The hexanucleotide repeat expansion, GGGGCC (G4C2), within the first intron of the C9orf72 gene is known to be the most common genetic cause of both amyotrophic lateral sclerosis (ALS) and frontotemporal dementia (FTD). The G4C2 repeat expansions, either DNA or RNA, are able to form G-quadruplexes which induce toxicity leading to ALS/FTD. Here, we present the first crystal structures of an eight-layer parallel tetrameric G-quadruplex formed by two repeats of C9orf72 HRE DNA, d(G4C2)2, in Ba2+ and K+ solution, named as d(G4C2)2-Ba and d(G4C2)2-K respectively. Two d(G4C2)2 oligonucleotides form a parallel propeller-type dimeric G-quadruplex which stacks in a 5′-to-5′ arrangement making up a tetramer.

The crystal structure of d(G4C2)2-Ba in C2221 space group was solved by Ba-SAD method to 1.60 Å resolution. For the structure of d(G4C2)2-Ba (C2221), the asymmetric unit contains six chains, A–F. Intriguingly, two d(G4C2)2 oligonucleotides form a parallel-stranded dimeric G-quadruplex unit (i.e. chains A/B, chains C/D, chains E/F) which is composed of four G-tetrads connected by two CC double-chain-reversal loops. Specifically, chains A/B and their crystallographically symmetric molecules (chains Asym/Bsym) form a parallel-stranded tetrameric eight-layer G-quadruplex termed as Form-1/7 with the G1 base in one dimeric block stacks (i.e. chains A/B) with the G7 base in the opposite dimeric block (i.e. chains Asym/Bsym). While another two identical parallel-stranded tetrameric G-quadruplexes are formed by the chains C/D with their crystallographically symmetric molecules (chains Csym/Dsym) or chains E/F with their crystallographically symmetric molecules (chains Esym/Fsym). Both of them are named as Form-1/1 as the G1 base of one dimeric block (i.e. chains C/D or chains E/F) stacks on the G1 base of another dimeric block (i.e. chains Csym/Dsym or chains Esym/Fsym). The electron density was well defined for the four equal-spaced Ba2+ ions lying along the axis within the central core of the eight-layer tetrameric G-quadruplex in Form-1/7 and Form-1/1. Each of them is coordinated to eight neighbouring guanine O6 atoms at a distance of ∼2.7 Å, featuring an anti-prismatic coordination environment, which mimics those of monovalent potassium ions in DNA G-quadruplexes. Interestingly, an additional Ba2+ ion is positioned between two adjacent dimeric G-quadruplexes (formed by chains A/B and chains C/D, respectively) in the asymmetric unit. Interestingly, the C11 and C12 bases from two isolated chains, chains A and F, form a C·C+•C·C+ quadruple base pair which stacks on a G-tetrad layer of Form-1/7, G4·G10·G4′·G10′, belonging to the neighbouring tetrameric G-quadruplex.

>GGGGCCGGGGCC[6x]Functional tau is most abundant in neuronal axons where it binds to microtubules, assists microtubule assembly, and is essential for the structural integrity of neurons and for axonal transport. Here, we identify a new amyloidogenic segment, PAM4 (Polymorphic AMyloid segment in repeat 4), encompassing residues 350–362 of R4, and show that it self-assembles into amyloid fibrils. Cryo-EM revealed that PAM4 fibrils are highly polymorphic, and, remarkably, that the polymorphs formed by this segment in isolation recapitulate the conformations that PAM4 adopts in polymorphs from different human tauopathies. In all cases, the folds share a C-terminal β-strand (residues 358–362) but differ in the way they orientate the N-terminus about an intermediary GS-bend (residues 355–356).

We also determined the structure of PAM4 amyloid fibrils formed by a lower purity (92%) peptide batch. Two-dimensional (2D) classification revealed that this peptide batch also formed multiple fibril polymorphs, with three distinct PAM4 fibril structures that could be determined to high resolution. The most abundant polymorph, PAM4 Type 2 (representing 28% of the total population), was resolved to a resolution of 2.8 Å. This polymorph has six peptide subunits per layer with a helical twist and rise of 358.55° and 4.8 Å, respectively, corresponding to a crossover distance of 60 nm. The resolution of the maps, in combination with liquid chromatography-mass spectrometry (LCMS) data, facilitated the identification of an adduct coming from a minor population of the peptide containing an N-terminal Fmoc protection group from peptide synthesis (~7.4%). Similarly, stacked protected N-termini pack at the protofibril interfaces of each of the three fibril structures with the C-termini extending towards the anterior fibril surface, which could potentially explain the additional structural morphologies resolved in the presence of the Fmoc protection group. Interestingly, the folds were interchangeable within the different fibril types, with Type 1 contaning FoldA and B, Type 2 fibrils containing FoldB, C and D, and Type 3 and Type 4 fibrils containing FoldC and D. FoldB PAM4, which has a flipped N-terminal compared to the previous fold, perfectly matches the 4R PSP-derived tau fibril cores and shows a C-terminal mismatch to the 3R PiD tau polymorph. Finally, FoldD PAM4 matches R2:R3:R4 (4R) tau strains that are associated with corticobasal degeneration (CBD) and argyrophilic grain disease (AGD). Specifically, the FoldC conformation of PAM4 stabilised by the K353-D358 salt-bridge is also found in tau C-fold protofilament polymorphs linked to Alzheimer’s disease (AD), Gerstmann-Sträussler-Scheinker (GSS), primary age-related tauopathy (PART) and cerebral amyloid angiopathy (CAA), while showing reasonable fit to chronic traumatic encephalopathy (CTE) polymorphs.

>[18x]XVQSKIGSLDNITHX> GPMAQQKVVLKVPTMTDEKTKQKAIEAVADIYGIDSIAADLKDNK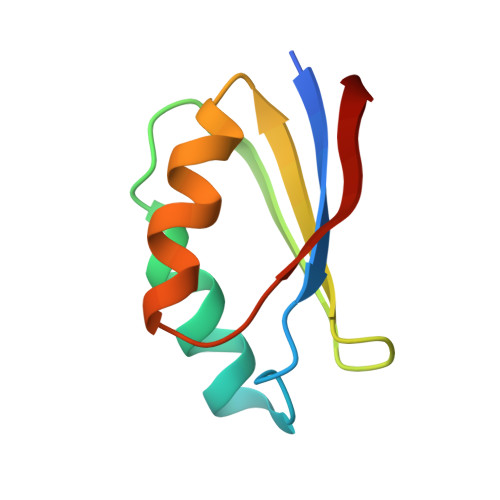MTIIGDMDTVEIAKKLRKIGKIDIVSVGPA>MHHHHHHHHENLYFQGKTEVAPGVHHVHPLPDSVPESEDLFAPPPRMQGKEGRPKPHIGPNYESYVKEWAKTVGPNSDEWWAAKARETLDWYDDFKTVRAGGFEHGDVQWFPEGTLNAAYNCLDRHYYKNPKKTAIIYEADEPSESREVSYEELMQETCRVANVLKSYGVKKGDAVSIYLPMTWQAAAAFLACARIGAIHSAVFAGFSAESLRDRVNDCECKVLITTDEGRRGGKTIATKQIVDAALQQCPLVENVLVLRRTGNKVPMTEGRDKWWDEECAKMPAYCPCERMASEDPLFILYTSGSTGKPKGVVHSTAGYLLGTALTLKYVFDAHPDDRFACMADIGWITGHSYIIYGPLANGITTAVFESTPVYPTPSRYWDFVDKWKATQLYTAPTAIRLLRRMGEDHVKNHDLSSLRVLGSVGEPINPEAWHWYNDFAGKNQCAIVDTYWMTETGSISIAPLPGAISTKPGSATFPFFGMDVDIIDPQTGQVLEGNDVEGVLVARRPWPSIARTVYRDHKRYLETYMKPYPGYFFFGDGAARDYDGYMWIKGRVDDVINVSGHRLSTAEVESALILHKGVAETAVVGCADDLTGQAVYAFVTMKPEFDLKATKEADLSKELAIQVRKVIGPFAAP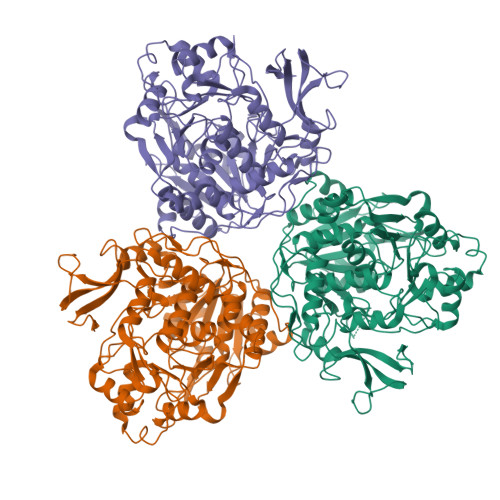KKIYLVSDLPKTRSGKIMRRVLRKIVAGEGDQLGDLSSIADPQIVEEVKQKVTGSA[3x]> GGSMATNENLPEIMTKLWDSKAQGEQEELHLLKGSDCNLTIDITEKCLRLAQRSAYQLHTETSATKRIQKFFLLGSLNINKDDRVIINIDRFDPGRIIDRKEGNKSLHVPTAVIPGDVIIPLSMQLACLGSEGVSPFSISEYYDAFQTLTKNLKLSCDSVDIKDMLSLKIHATYYVDSDEISINVTSGVVVPSALITAVPILPVSIVPTALARSLSGPLHLSNFQDTQKSGYVAINNSHNLLLVLDSDPKLSSI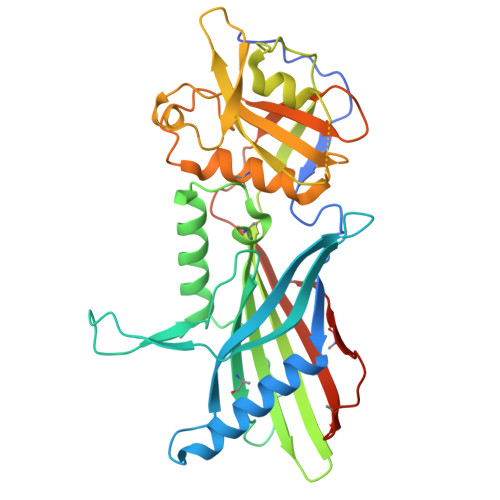PLVGIWVDGVISIHHPYVWSACMRYLYSQRLTNKIRDGSTGFILVLYTQTRPKPEFWECSFSGKSDKFLYCQASDDIFMEKVAKTRNEYMRLQLVPNEFGENLYFQ>MGTGKGFGVKCVSLKMAKGLTISLLFGWALMAGSSALAATVTDMAGRTVTIPAKVERILLGEGRLFYAVSLLEGNKPLDRIVGWQGDFRKLDPQTYAIYKAKFPQIDQIPLIGNTTADSISPEKVLTLNPDIAIFGLSGHGPGKGSELVKQLEKAGVPVVFVDFRNSPLKNTLPSMRLLGKALHREQQAENYINFYQDNVDKVTDITNKIPEDKKPSVFIELRAGASEECCGTAGKGNMGDFIDQAGGNNIAKNLLPGSLGTVNLEKVLAAKPDIYIA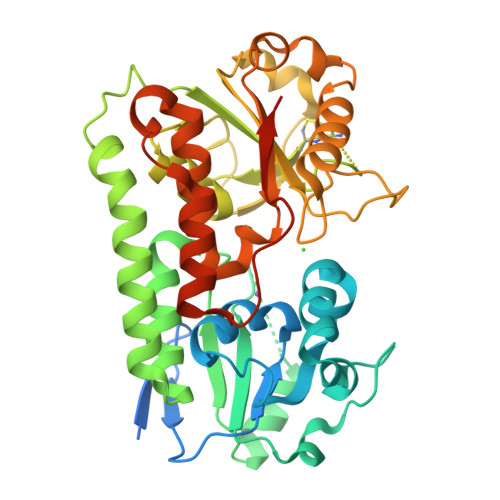SGGKSPGSDAPGVVLGAQVTPEQAQASLQKILGRKGINTLSAVNTGHSYAIWHNYYNSPYNVLAIQSFAKWFYPEQFADLDPKKTMDSLYSQFLAVEPSGTYWIEAKRELDLEHHHHHHHHHH[2x]>AECSVDIQGNDQMQFNTNAITVDKSCKQFTVNLSHPGNLPKCVMGHNWVLSTAADMQGVVTDGMASGLDKDYLKPDDS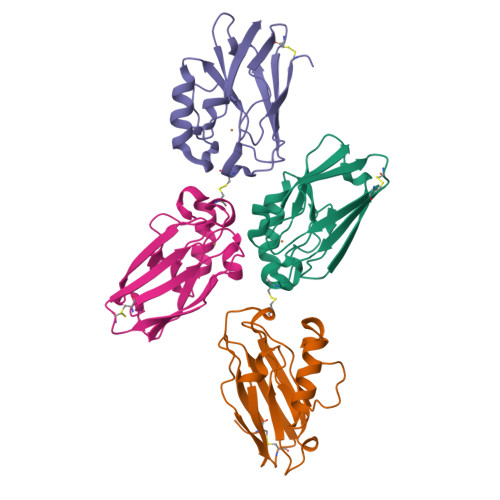RVIAHTKLIGSGEKDSVTFDVSKLKEGEQYMFFCTFPGHSALMKGTLTLK[12x]>[2x]MLSNSQGQSPPVPFPAPAPPPQPPTPALPHPPAQPPPPPPQQFPQFHVKSGLQIKKNAIIDDYKVTSQVLGLGINGKVLQ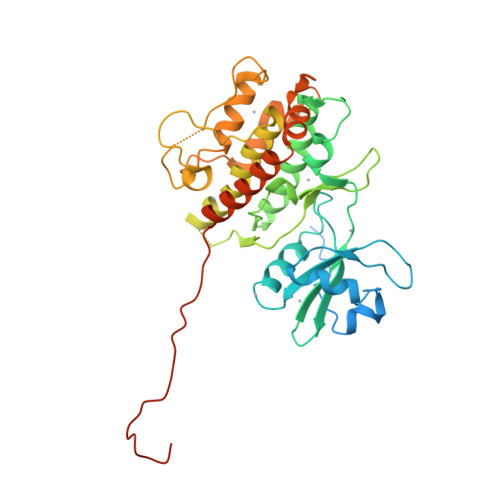IFNKRTQEKFALKMLQDCPKARREVELHWRASQCPHIVRIVDVYENLYAGRKCLLIVMECLDGGELFSRIQDRGDQAFTEREASEIMKSIGEAIQYLHSINIAHRDVKPENLLYTSKRPNAILKLTDFGFAKETTSHNSLTTPCYTPYYVAPEVLGPEKYDKSCDMWSLGVIMYILLCGYPPFYSNHGLAISPGMKTRIRMGQYEFPNPEWSEVSEEVKMLIRNLLKTEPTQRMTITEFMNHPWIMQSTKVPQTPLHTSRVLKEDKERWEDVKEEMTSALATMRVDYEQIKIKKIEDASNPLLLKRRKKARALEAAALAH2-hydroxyethyl 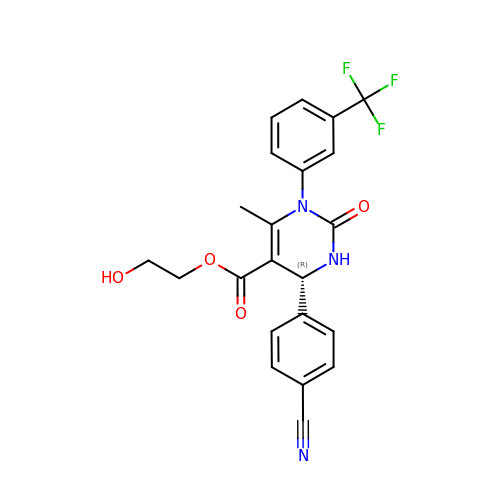(4R)-4-(4-cyanophenyl)-6-methyl-2-oxo-1-[3-(trifluoromethyl)phenyl]-1,2,3,4-tetrahydropyrimidine-5-carboxylate | C22 H18 F3 N3 O4 | XERLAFZWYABQAT-LJQANCHMSA-N> MGYAHPEVLVSTDWVQEHLEDPKVRVLEVDEDILLYDTGHIPGAQKIDWQRDFWDPVVRDFISEEEFAK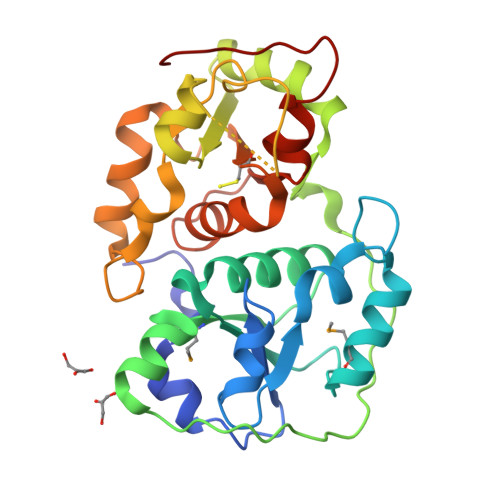LMERLGISNDTTVVLYGDKNNWWAAYAFWFFKYNGHKDVRLMNGGRQKWVEEGRPLTTEVPSYPPGRYEVPYRDESIRAYRDDVLEHIIKVKEGKGALVDVRSPQEYRGELTHMPDYPQEGALRAGHIPGAKNIPWAKAVNPDGTFKSAEELRALYEPLGITKDKDIVVYCRIAERSSHSWFVLKYLLGYPHVKNYDGSWTEWGNLVGVPIAKGEE>[2x]MGLEKTVKEKLSFEGVGIHTGEYSKLIIH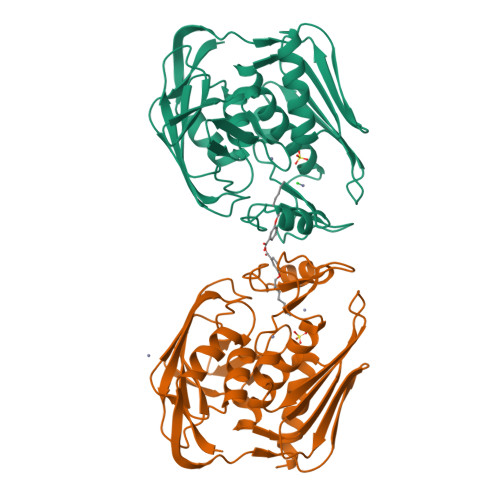PEKEGTGIRFFKNGVYIPARHEFVVHTNHSTDLGFKGQRIKTVEHILSVLHLLEITNVTIEVIGNEIPILDGSGWEFYEAIRKNILNQNREIDYFVVEEPIIVEDEGRLIKAEPSDTLEVTYEGEFKNFLGRQKFTFVEGNEEEIVLARTFAFDWEIEHIKKVGLGKGGSLKNTLVLGKDKVYNPEGLRYENEPVRHKVFDLIGDLYLLGSPVKGKFYSFRGGHSLNVKLVKELAKKQKLTR> K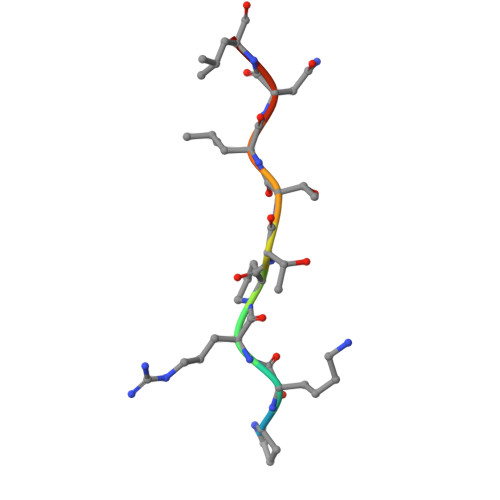PKRPTTLNLF>[2x]MHHHHHHTSLYKKAG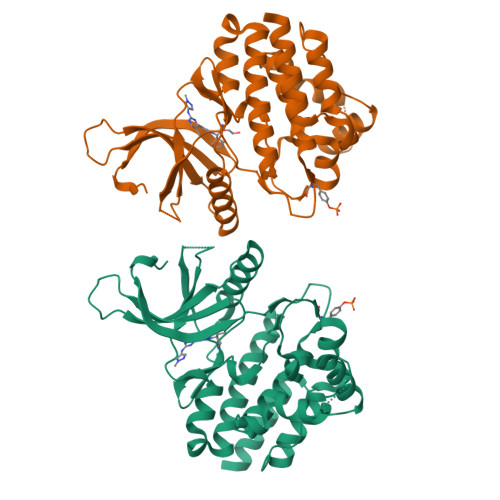FLVPRGSEDRDPTQFEERHLKFLQQLGKGNFGSVEMCRYDPLQDNTGEVVAVKKLQHSTEEHLRDFEREIEILKSLQHDNIVKYKGVCYSAGRRNLKLIMEYLPYGSLRDYLQKHKERIDHIKLLQYTSQICKGMEYLGTKRYIHRDLATRNILVENENRVKIGDFGLTKVLPQDKEYYKVKEPGESPIFWYAPESLTESKFSVASDVWSFGVVLYELFTYIEKSKSPPAEFMRMIGNDKQGQSIVTHLIELLKNNGRLPRPDGCPDEIYMIMTECWNNNVNQRPSFRDLALRVDQIRDQMAG> SGVDDDMACHKIP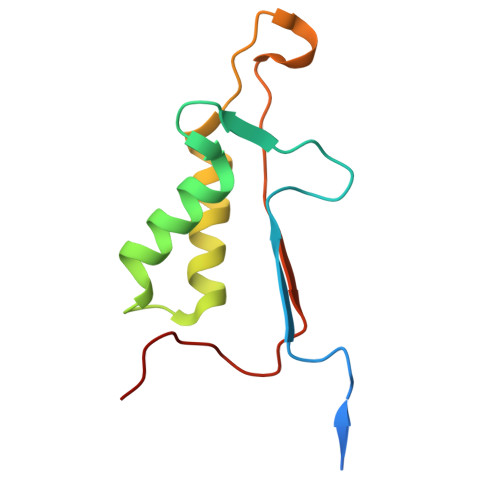VEADFLYAYSTAPGYYSWRNSKDGSWFIQSLCAMLKQYADKLEFMHILTRVNRKVATEFESFSFDATFHAKKQIPCIVSMLTKELYFYHH However, applying it to GPCRs without signaling proteins remains challenging because most receptors lack structural features in their soluble domains to facilitate image alignment. Although integral membrane proteins like GPCRs are challenging to crystallize, a highly successful strategy is to engineer a fusion protein replacing the third intracellular loop (ICL3), located between transmembrane helices 5 (TM5) and 6 (TM6), so that the inserted fusion protein can mediate crystal contacts. We use two model systems for this interrogation, the adenosine A2A receptor (A2AR) and the Smoothened receptor (SMO), both of which have previously been interrogated by X-ray crystallography and cryo-EM. By exploring various fusion strategies, we determine a 3.4 Å resolution structure of antagonist-bound inactive A2AR in detergent micelle and a 3.7 Å structure of unliganded inactive SMO in a lipidic environment.

We designed two different constructs, mSMO-PGS1, in which the PGS domain is inserted to SMO after position 441 on ICL3 and before position 445 on TM6, and mSMO-PGS2, in which PGS has inserted one and a half helical turns (five amino acids) up towards in TM6. The reconstruction of mSMO-PGS2 is, surprisingly, different from the AlphaFold prediction but reaches a significantly better resolution of 3.7 Å. Unlike the AlphaFold prediction, the PGS is oriented beneath TM bundle without a continuous helix between TM6 of mSMO and the C terminus of PGS, but a contorted loop that allows the PGS domain to directly interact with the mSMO 7TM bundle. At the interface of mSMO and PGS, a hydrophobic loop of PGS (F1124, L1126, L1129, I1149, and F1195) contacts hydrophobic residues at the base of TM3 and TM5 (F347, L350, I433, and L440). This unpredicted hydrophobic interaction with the intracellular side of mSMO likely stabilized the orientation of PGS relative to mSMO. We surmised that this interaction enabled a rigid attachment of PGS to mSMO and facilitated a higher resolution reconstruction of the mSMO 7TM domain. Our cryo-EM structure of mSMO in saposin nanodisc enabled modeling of the 7TM and linker domain (LD), which connects the extracellular CRD with the 7TM domain. The bulk of the SMO CRD is poorly resolved in our map, except for two small density fragments in the region connecting the 7TM to the CRD, one of which has the appearance of a short helix. In comparison with previous structures of SMO, our structure of apo SMO resembles the inactive SMO, with an overall RMSD of 0.75 Å in the 7TM region and a conformation of TM5 and TM6 that is consistent with an inactive receptor. Consistent with an apo state, this pocket is empty in our structure without the obvious density of any bound ligand or sterols.

> WSHPQFEKENLYFQSPRLLSHCGRAAHCEPLRYNVCLGSALPYGATTTLLAGDSDSQEEAHGKLVLWSGLRNAPRCWAVIQPLLCAVYMPKCENDRVELPSRTLCQATRGPCAIVERERGWPDFLRCTPDHFPEGCPNEVQNIKFNSSGQCEAPLVRTDNPKSWYEDVEGCGIQCQNPLFTEAEHQDMHSYIAAFGAVTGLCTLFTLATFVADWRNSNRYPAVILFYVNACFFVGSIGWLAQFMDGARREIVCRADGTMRFGEPTSSETLSCVIIFVIVYYALMAGVVWFVVLTYAWHTSFKALGTTYQPLSGKTSYFHLLTWSLPFVLTVAILAVAQVDGDSVSGICFVGYKNYRYRAGFVLAPIGLVLIVGGYFLIRGVMTLFSIKSNHPGLLGIDCSFWNESYLTGSRDERKKSLLSKFGMDEGVTFMFIGRFDRGQKGVDVLLKAIEILSSKKEFQEMRFIIIGKGDPELEGWARSLEEKHGNVKVITEMLSREFVRELYGSVDFVIIPSYFEPFGLVALEAMCLGAIPIASAVGGLRDIITNETGILVKAGDPGELANAILKALELSRSDLSKFRENCKKRAMSFSDQARMDIRLAKNETMLRLGIFGFLAFGFVLITFSCHFYDFFNQAEWERSFRDYVLCQANVTIGLPTKKPIPDCEIKNRPSLLVEKINLFAMFGTGIAMSTWVWTKATLLIWRRTWCRLTGHSDDEPKR>MRGSHHHHHHGRSLNPLSTPQFDSTDETPASYNLAVRRAAPAVVNVYNRGLNTNSHNQLEIRTLGSGVIMDQRGYIITNKHVINDADQIIVALQDGRVFEALLVGSDSLTDLAVLKINATGGLPTIPINARRVPHIGDVVLAIGNPYNLGQTITQGIISATGRIGLNPTGRQNFLQTDASINHGNSGGALVNSLGELMGINTLSFDKSNDGETPEGIGFAIPF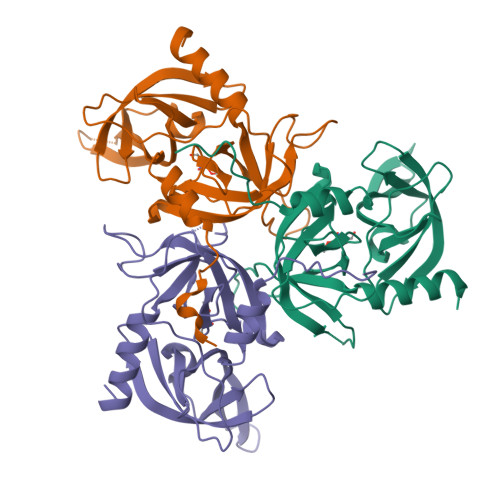QLATKIMDKLIRDGRVIR[9x]>[2x]YRPISQGVSDLVGLPNQICLQKTTSTILKPRLISYTLPINTREGVCITDPLLAVDNGFFAYSHLEKIGSCTRGIAKQRIIGVGEVLDRGDKVPSMFMTNVWTPPNPSTIHHCSSTYHED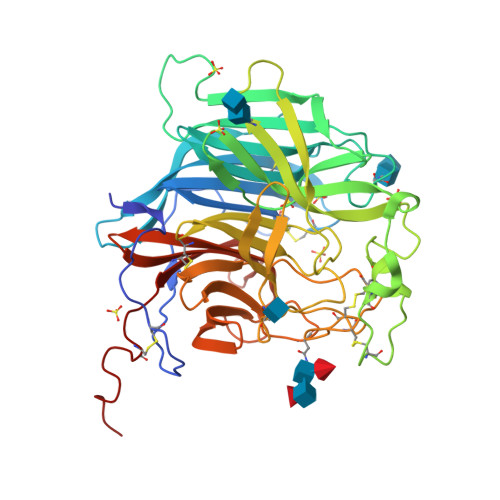FYYTLCAVSHVGDPILNSTSWTESLSLIRLAVRPKSDSGDYNQKYIAITKVERGKYDKVMPYGPSGIKQGDTLYFPAVGFLPRTEFQYNDSNCPIIHCKYSKAENCRLSMGVNSKSHYILRSGLLKYNLSLGGDIILQFIEIADNRLTIGSPSKIYNSLGQPVFYQASYSWDTMIKLGDVDTVDPLRVQWRNNSVISRPGQSQCPRFNVCPEVCWEGTYNDAFLIDRLNWVSAGVYLNSNQTAENPVFAVFKDNEILYQVPLAEDDTNAQKTITDCFLLENVIWCISLVEIYDTGDSVIRPKLFAVKIPAQCSESGRGLVPR>MIRISNKIKTLLAMLSFVQVTSGCDATVQDIIIDTDPGVEIGNNDYYTWCKETLSVIDKDLKISGTHSYYENQDRSQVSFIWGNIFLLYTYTEGISLSKSEWSDALMNCFLNFDNYWHPNYKGIAGYATLPTSAEKVPDRFYDENGWTAIGLCDAYLATQNNSYLEKAKGALAFSLSGEDNVLGGGIYFQETFVSLPVQKNTICSAVTMLSCMKLYEITQDRQYLDAAIRINDWTVENLLDKSDNLLWDAKMVADGSVNTQKWSYNAGFMIRSWLKMYQATKDEKYLSQAKATLASSEAKWYNSINGALNDPGYFAFSIIDSWFDMYDTDKNTVWLTKAFHAINFIHNKLRDGNGRYPEHWGTPTTSNLEKYDLRFSTVAAYMYMRAANYKRILND[2x]

By comparison, early studies have shown GH76 enzymes to be far more specific, with activity only detectable against the extended α-1,6-mannoside backbone present in yeast α-mannans. In this paper, we present the crystal structure, determined by SAD phasing of a selenomethionine derivative, of one such GH76 enzyme from Bt, BT2949. Furthermore, we show that despite poor homology at the primary amino-acid level, the tertiary structure of BT2949 appears to be well conserved in other GH76 family members. These enzymes form a long trough-like structure, which is consistent with a requirement to accommodate extended polysaccharides such as α-mannan.

Initial merging of the data with AIMLESS in space group P212121 appeared satisfactory (systematic absence probability of ≥0.98 for three 21 screw axes); however, the structure could not be solved after several attempts at SAD phasing, with poor contrast and mapCC (correlation coefficient) between the two possible hands for the structure. Subsequent reprocessing of the data in P22121 allowed facile phasing of the selenium substructure and model building of two complete BT2949 molecules. The crystals of BT2949 belonged to the orthorhombic space group P22121 (unit-cell parameters a = 81, b = 121, c = 126 Å, α = β = γ = 90°) with two protein molecules present in each asymmetric unit (molecules A and B appear identical, with an average r.m.s.d of 0.07 Å across matching Cα positions). The final atomic model for each monomer spans a continuous peptide chain comprising residues Pro37–Asn395 (residues 1–22 form a signal peptide and were removed in this construct to allow soluble gene expression).2-[(1~{R})-3-[bis(fluoranyl)methoxy]-1-[4-(3-methyl-1,2,3-triazol-4-yl)pyrazol-1-yl]propyl]-5-[3-chloranyl-6-(4-chloranyl-1,2,3-triazol-1-yl)-2-fluoranyl-phenyl]-1-oxidanyl-pyridine 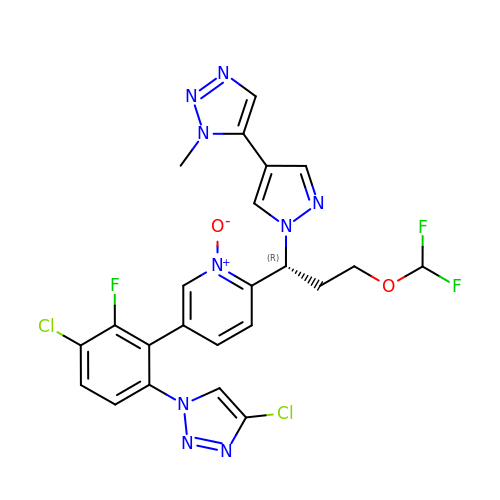| C23 H18 Cl2 F3 N9 O2 | BETDGMHNHGHORO-MRXNPFEDSA-N>SIGTRWAVLIAGSKGYHNYRHQADVCHMYQILRKGGVKDENIIVFMYDDIAYNESNPFPGIIINKPGGENVYKGVPKDYTGEDINNVNFLAAILGNKSAIIGGSGKVLDTSPNDHIFIYYAXGAPGKIGMPSKPYLYADDLVDTLKQKAATGTYKSMVFYVEACNAGSMFEGLLPEGTNIYAMAASNSTEGSWITYCPGTPDFPPEFDVCLGDLWSITFLEDCDAHNLRTETVHQQFELVKKKIAYASTVSQYGDIPISKDSLSV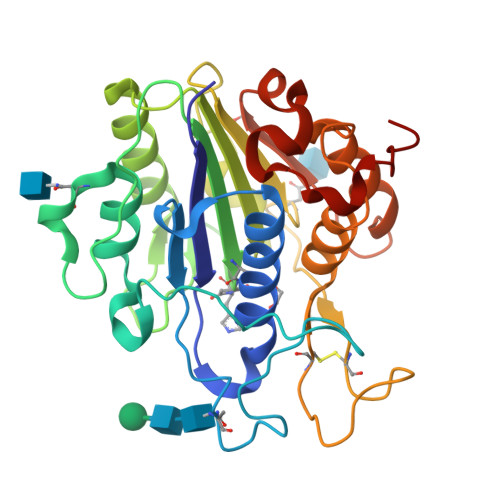YMGTDPANDNRTFVDEN[2x]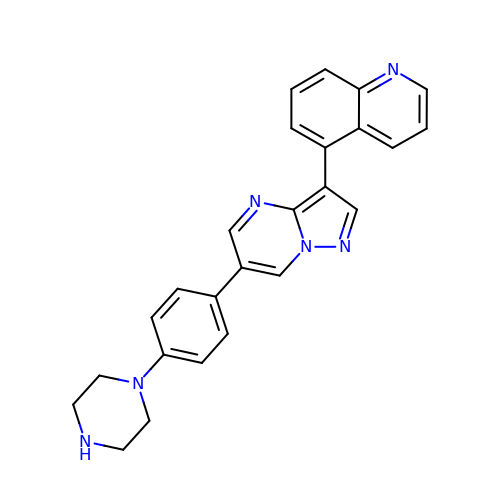5-[6-(4-piperazin-1-ylphenyl)pyrazolo[1,5-a]pyrimidin-3-yl]quinoline | C25 H22 N6 | BBDGBGOVJPEFBT-UHFFFAOYSA-N> GSHMMRNELEEMQR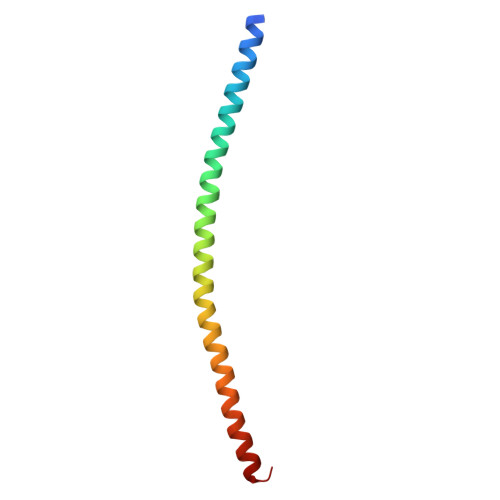RADQLADESLESTRRMLQLVEESKDAGIRTLVMLDEQGEQLDRVEEGMNHINQDMKEAEKNLKDLGW> GSSHHHHHH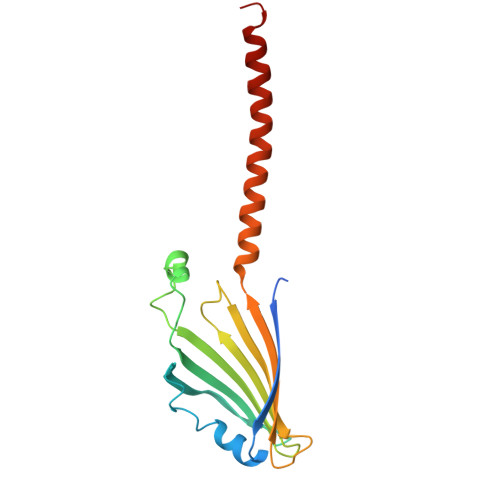SDQMVKYFLGQSVLRSSWDQVFAAFWQRYPNPYSKHVLTEDIVHREVTPDQKLLSRRLLTVTNRMPRWAERLFPANVAHSVYVLEDSIVDPQNQTMTTFTWNINHARLMVVEERSVYSVNSDNSGWTEIRREAWVSSSLFGVSRAVQEFGLARFKSNVTKTMKGFEYILAKLQGEA>GDSIEDKNARVIELIAAYRNRGHLMADIDPLRLDNTRFRSHPDLDVNSHGLTLWDLDREFKVDGFAGVQRKKLRDILSVLRDAYCRHVGVEYTHILEPEQQRWIQERVETKHDKPTVAEQKYILSKLNAAEAFETFLQTKYVGQKRFSLEGAETVIPMMDAVIDQCAEHGLDEVVIAMPHRGRLNVLANIVGKPYSQIFSEFEGNLNPSQAHGSGDVKYHLGATGTYIQMFGDNDIEVSLTANPSHLEAVDPVLEGLVRAKQDLLDTGEEGSDNRFSVVPLMLHGDAAFAGQGVVAETLNLALLRGYRTGGTIHIVVNNQIGFTTAPTDSRSSEYCTDVAKMIGAPIFHVNGDDPEACAWVARLAVDFRQAFKKDVVIDMLCYRRRGHNEGDDPSMTQPYMYDVIDTKRGSRKAYTEALIGRGDISMKEAEDALRDYQGQLERVFNEVRELEKHEIEPSESVEADQQIPSKLATAVDKAMLQRIGDAHLALPEGFTVHPRVRPVLEKRREMAYEGRIDWAFAELLALGSLIAEGKLVRLSGQDTQRGTFTQRHAVIVDRKTGEEFTPLQLLATNPDGTPTGGKFLVYNSALSEFAAVGFEYGYSVGNPD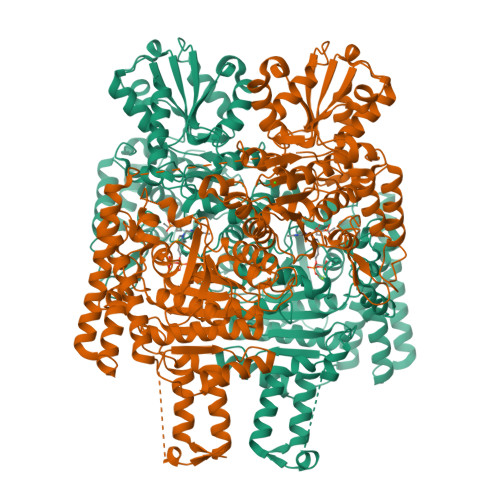AMVLWEAQFGDFVNGAQSIIDEFISSGEAKWGQLSDVVLLLPHGHEGQGPDHTSGRIERFLQLWAEGSMTIAMPSTPANYFHLLRRHGKDGIQRPLIVFTPKSMLRNKAAVSDIRDFTESKFRSVLEEPMYTDGEGDRNKVTRLLLTSGKIYYELAARKAKENREDVAIVRIEQLAPLPRRRLAETLDRYPNVKEKFWVQEEPANQGAWPSFGLTLPEILPDHFTGLKRISRRAMSAPSSGSSKVHAVEQQEILDTAFG[4x]Baricitinib | C16 H17 N7 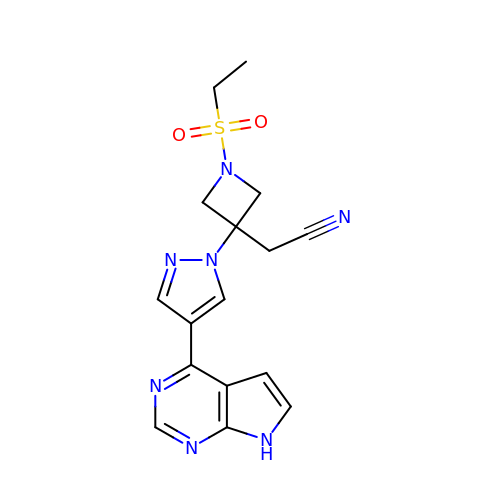O2 S | XUZMWHLSFXCVMG-UHFFFAOYSA-N> SNAMSKSNQKIASIEQLSNNEGIISALAFDQRGALKRMMAKHQTEEPTVAQIEQLKVLVAEELTQYASSILLDPEYGLPASDARNKDCGLLLAYEKTGYDVNAKGRLPDCLVEWSAKRLKEQGANAVKFLLYYDVDDAEEINIQKKAYIERIGSECVAEDIPFFLEVLTYDDNIPDNGSVEFAKVKPRKVNEAMKLFSEPRFNVDVLKVEVPVNMKYVEGFAEGEVVYTKEEAAQHFKDQDAATHLPYIYLSAGVSAELFQETLKFAHEAGAKFNGVLCGRATWSGAV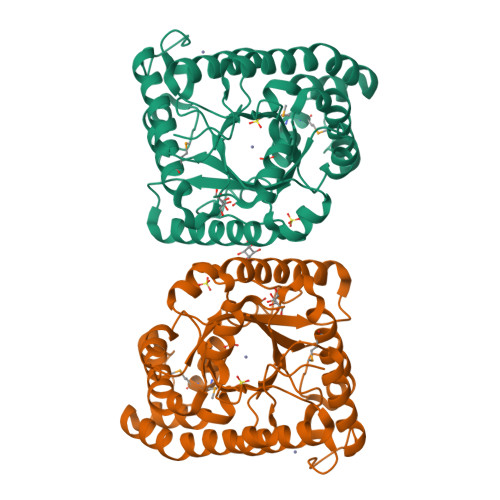QVYIEQGEDAAREWLRTTGFKNIDDLNKVLKDTATSWKQRK>[2x]NLKPVDAMQCFDCHTQIEDMHTVGKHATVNCVHCHDATEHVETASSRRMGERPVTRMDLEACATCHTAQFNSFVEVRHESHPRLEKATPTSRSPMFDKLIAGHGFAFEHAEPRSHAFMLVDHFVVDRAYGGRFQFKNWQKVTDGMGAVRGAWTVLTDADPESSDQRRFLSQTATAANPVCLNCKTQDHILDWAYMGDEHEAAKWSRTSEVVEFARDLNHPLNCFMCHDPHSAGPRVVRDGLINAVVDRGLGTYPHDPVKSEQQGMTKVTFQRGREDFRAIGLLDTADSNVMCAQCHVEYNCNPGYQLSDGSRVGMDDRRANHFFWANVFDYKEAAQEIDFFDFRHATTGAALPKLQHPEAETFWGSVHERNGVACADCHMPKVQLENGKVYTSHSQRTPRDMMGQACLNCHAEWTEDQALYAIDYIKNYTHGKIVKSEYW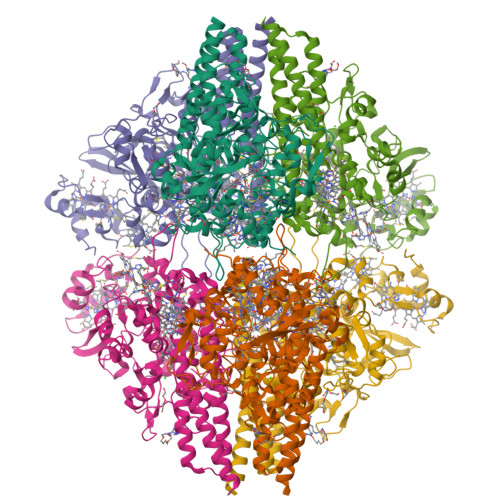LAKMIDLFPVAKRAGVSEDVLNQARELHYDAHLYWEWWTAENSVGFHNPDQARESLMTSISKSKEAVSLLNDAIDAQVAS>[2x]SHMSEISRVALFGKLNSLAYKAIEAATVFCKLRGNPYVELVHWFHQILQLPDSDLHQIVRQSGIDPARLAKDLTEALDRLPRGSTSITDLSSHVEEAVERGWVYGSLMFGESQVRTGYLVIGILKTPSLRHALTGLSAEFAKLKVEALTERFDEYVGASPENG

The type VI secretion system (T6SS) is a bacterial nanomachine for the transport of effector molecules into prokaryotic and eukaryotic cells. It involves the assembly of a tubular structure composed of TssB and TssC that is similar to the tail sheath of bacteriophages. The AAA+ ATPase ClpV disassembles the contracted sheath, which resets the systems for reassembly of an extended sheath that is ready to fire again. The interaction of TagJ/HsiE with the sheath as well as with ClpV suggests an alternative mode of disassembly in which HsiE recruits the ATPase to the sheath.

In this study, we resolved the crystal structure of the N-terminal domain of Pseudomonas aeruginosa ClpV1 and observed structural alterations in the hydrophobic groove. The asymmetric unit contains two copies of ClpV1-N in nearly identical conformations (r.m.s. deviation for all Cα atoms of 0.5 Å). The overall structure of ClpV1-N is similar to that of the Vibrio ClpV-N, with matching secondary structure elements and an r.m.s. deviation of 1.6 Å for 121 equivalent Cα atoms. Both structures possess an N-terminal helix α0 that distinguishes ClpV-type ATPases from other Hsp100 ATPases (e.g. ClpA). The residues lining the VipB binding groove in ClpV-N are partially conserved in ClpV1-N. For example, Ile10 and Phe87 lie at the bottom of the groove. The corresponding residues in ClpV1-N are Phe10 and Leu88. The two aliphatic residues Leu6 and Ala86, which sit at the top of the groove in Vibrio ClpV-N, are replaced by large residues of opposite charge in ClpV1-N (i.e. Arg6 and Asp87). In one of the two ClpV1-N molecules in the asymmetric unit, these residues form a salt bridge across the groove, whereas in the other, they point into the groove. Both conformations not only diminish the hydrophobic character of the groove but also are incompatible with binding of an α-helix, as observed in V. cholerae. Consistent with the altered conformation of the binding groove, we were unable to obtain a complex of ClpV1-N bound to a peptide corresponding to the N terminus of HsiC1.> GPGSMACLSRIDANLLQYYEKPEPNNTVDLYVSNNSNNNGLKEGDKSISTPVPQPYGSEYSNCLLLSNSEYICYHFSSRSTLLTFYPLSDAYHGKTINIHLPNASMNQRYTLTIQEVEQQLLVNVILKDGSFLTLQLPLSFLFSSANTLNGEWFHLQNPYDFTVRVPHFLFYVSPQFSVVFLEDGGLLGLKKVDGVHYEPLLFNDNSYLKSLTRFFSRSSKSDYDSVISCKLFHERYLIVLTQNCHLKIWDLTSFTLIQDYDMVSQSDSDPSHFRKVEAVGEYLSLYNNTLVTLLPLENGLFQMGTLLVDSSGILTYTFQNNIPTNLSASAIWSIVDLVLTRPLELNVEASYLNLIVLWKSGTASKLQILNVNDESFKNYEWIESVNKSLVDLQSEHDLDIVTKTGDVERGFCNLKSRYGTQIFERAQQILSENKIIMAHNEDEEYLANLETILRDVKTAFNEASSITLYGDEIILVNCFQPYNHSLYKLNTTVENWFYNMHSETDGSELFKYLRTLNGFASTLSNDVLRSISKKFLDIITGELPDSMTTVEKFTDIFKNCLENQFEITNLKILFDELNSFDIPVVLNDLINNQMKPGIFWKKDFISAIKFDGFTSIISLESLHQLLSIHYRITLQVLLTFVLFDLDTEI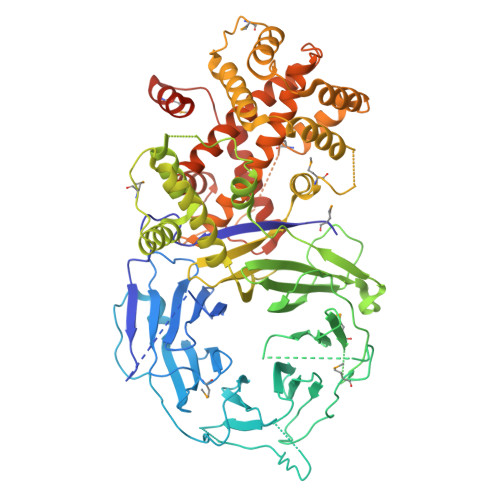FGQHISTLLDLHYKQFLLLNLYRQDKCLLAEVLLKDSSEFSFGVKFFNYGQLIAYIDSLNSNVYNASITENSFFMTFFRSYIIENTSHKNIRFFLENVECPFYLRHNEVQE>[2x]CVIFPVEIDVSQTIIRDCQVDKQTRELVYINKIMNTQLTKPVLMMFNISGP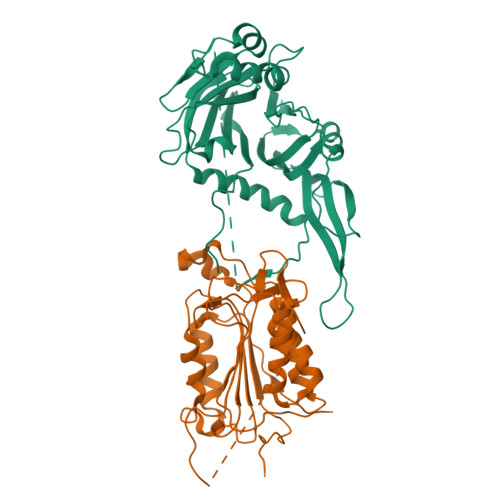IRSVTRKNNNLRDRIKSKVDEQFDQLERDYSDQMDGFHDSIKYFKDEHYSVSCQNGSVLKSKFAKILKSHDYTDKKSIEAYEKYCLPKLVDERNDYYVAVCVLKPGFENGSNQVLSFEYNPIGNKVIVPFAHEINDTGLYEYDVVAYVDSVQFDGEQFEEFVQSLILPSSFKNSEKVLYYNEASKNKSMIYKALEFTTESSWGKSEKYNWKIFCNGFIYDKKSKVLYVKLHNVTSALNKNVILNTIK;>[2x]LDKVYQMKSKPRGYCLIINNHNFAKAREKVPKLHSIRDRNGTHLDAGALTTTFEELHFEIKPHHDCTVEQIYEILKIYQLMDHSNMDCFICCILSHGDKGIIYGTDGQEAPIYELTSQFTGLKCPSLAGKPKVFFIQACQGDNYQKGIPVETDSEEQPYLEMDLSSPQTRYIPDEADFLLGMATVNNCVSYRNPAEGTWYIQSLCQSLRERCPRGDDILTILTEVNYEVSNKDDKKNMGKQMPQPTFTLRKKLVFPSD5-ethynyl-1-(beta-D-glucopyranosyl)pyrimidine-2,4(1H,3H)-dione | 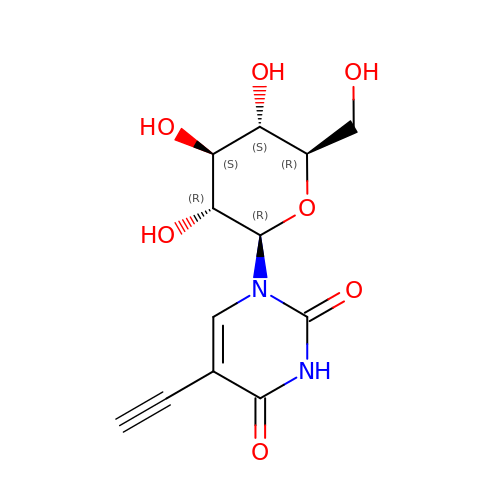C12 H14 N2 O7 | DSYJZEAWLKMMLW-ZBGLXGBJSA-N> KSAVT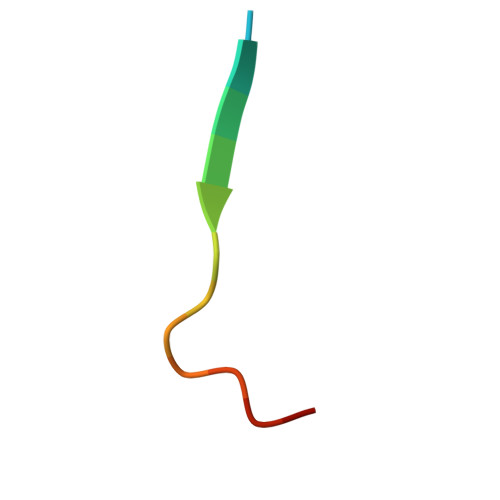TVVNPQYEGK>[2x]MTLLCGEIHYFRVPKHLWRDRLLKLKRAGGNCVSTYIPWNWHDPREKVVNFTDGTSQWHVASYYSRDLASFLELAGELGLRVIARPGPYICSEWDSGGHPNWIYTKAMRLRSLDPGYFKHVVEWYNSVLNILKPYVEREIVIGIQVENEYFWGNEKYIEKLAEIVEEK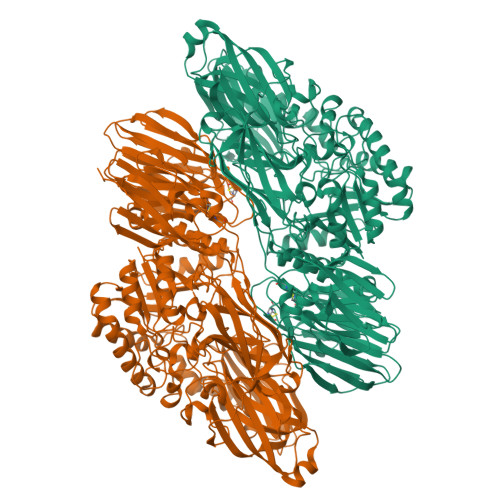LPGVLVFTNEDPYLTRIPNTIDLYPSPWDMRQFDDRLRSYLSSQPGLFKMIMELEGGWFKSSRYGYYPTNRLSIPPEWTEILLKTAVGMGLNNINIYMFHGGSNPGYYTAKYLASSYDFEACIREWGELSERYYRVKRVFTFLNGFQELVTSLKPGETVKTASTCSELLQRVGDHGKIAVLRNTGDNLCYQRLINRGEIIPMWTPIRVPPRYAKIVLLDLVVEGTPFKLVYTSGEALLMKRLGDTVVMIIYGDHGEYTETAVEVEGGVLDVDIQGDVLIRREGERAYLVVNHTHGEHLAIVKSTRGQNLLLIFTCRCRAEKTWIVDEDLVLISNIYYIGDSRIDEGKVVINAELDEDSCGRLLVVTSREIEAISLEDLDLDLTRLSKYVYATHIPLSMCRSGKNTYHPLEYRLLEDPVFHTLTSINPSSPLEKNGFYENGIYVYRLRLHLDKKQLGDLLDKHLALIGFSDYAVVSINNEYAGSGYHYIEMSADSLREGVNEVTVILESTGHPNDGLLYVPNGIYGGVYLGRVGEIRLYKWRKTGFEIPYGPGFDLAEFIANPEPVIKALQEQRSSTGETYSVDSPGLYITEFKVDDLSRHYVLDPGLEFYYNHYYRILLFVNKVYVGPLIGPIDITRYLKPGVNEVALLVEWGVVNPVIGVYQYKVDGEWFIQEGLHGLIEEWFRRSPRGETAEPPILLGDKAGRVIWVNTVIPYEKEPTSSSPVKLEVDFWGCRILVFVNGEFIGRISDDSPERELYVPETAVRRGLNNITLLAIVTSRSSGIRGLRLKETYVHERKEIVFKLGLTKLAAALEHHHHHH(3alpha,9beta,10alpha,13alpha)-30-cyclopropylidenelanost-7-en-3-ol | C33 H54 O | 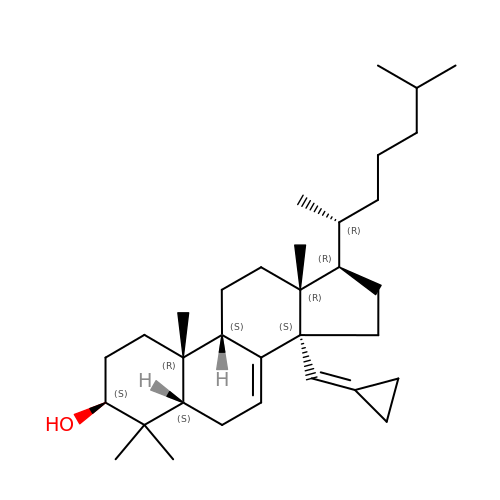JMJLBCGVSMHFQK-SIDBGHOXSA-N>MANVIKTVLTYQLDGSNRDFNIPFEYLARKFVVVTLIGVDRKVLTINTDYRFATRTTISLTKAWGPADGYTTIELRRVTSTTDRLVDFTDGSILRAYDLNVAQIQTMHVAEEARDLTTDTIGVNNDGHLDARGRRIVNLANAVDDRDAVPFGQLKTMNQNSWQARNEALQFRNEAETFRNQAEGFKNESSTNATNTKQWRDETKGFRDEAKRFKNTAGQYATSAGNSASAAHQSEVNAENSATASANSAHLAEQQADRAEREADKLENYNGLAGAIDKVDGTNVYWKGNIHANGRLYMTTNGFDCGQYQQFFGGVTNRYSVMEWGDENGWLMYVQRREWTTAIGGNIQLVVNGQIITQGGAMTGQLKLQNGHVLQLESASDKAHYILSKDGNRNNWYIGRGSDNNNDCTFHSYVHGTTLTLKQDYAVVNKHFHVGQAVVATDGNIQGTKWGGKWLDAYLRDSFVAKSKAWTQVWSGSAGGGVSVTVSQDLRFRNIWIKCANNSWNFFRTGPDGIYFIASDGGWLRFQIHSNGLGFKNIADSRSVPNAIMVENE[18x]

Escherichia coli bacteriophage T7, a member of Podoviridae, has been used as a model for understanding the DNA packaging mechanism common to tailed phages and related dsDNA viruses. The phages package genomic dsDNA into a round procapsid using the portal in complex with an ATP-dependent terminase complex as the motor. At the beginning of phage infection, the tail is responsible for receptor recognition, and the portal and tail act as a tunnel for DNA delivery into the host cytoplasm. Here, we determined structures of the DNA packaging intermediate and mature capsids of T7 using cryo-electron microscopy (cryo-EM) and symmetry-mismatch reconstruction.

Six trimers of the tail fiber gp17 N-termini anchoring to the adaptor-portal interface were clearly resolved. Each gp17 N-terminus is formed by a jelly-roll barrel and a 22-residue α-helix. The distal parts of the fibers, which are too flexible to be well resolved, were observed to radically extend back on the capsid shell at lower resolution.>MNDDVEFRYADFLFKNNNYAEAIEVFNKLEAKKYNSPYIYNRRAVCYYELAKYDLAQKDIETYFSKVNATKAKSADFEYYGKILMKKGQDSLAIQQYQAAVDRDTTRLDMYGQIGSYFYNKGNFPLAIQYMEKQIRPTTTDPKVFYELGQAYYYNKEYVKADSSFVKVLELKPNIY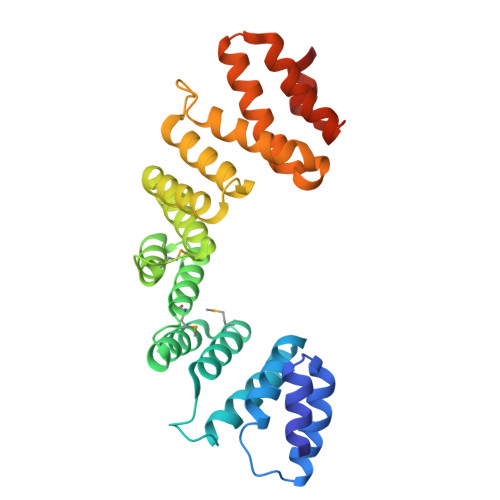IGYLWRARANAAQDPDTKQGLAKPYYEKLIEVCAPGGAKYKDELIEANEYIAYYYTINRDKVKADAAWKNILALDPTNKKAIDGLKMKLEHHHHHH[2x]>MKHHHHHHMHAGAQMDAESIEWKLTANLRNGPTFFQPLADSIEPLQFKLIGSDTVATAFPVFDTKYIPDSLINYLFKLFNLEIESGKTYPQLHSLTKQGFLNYWFHSFAVVVLQTDEKFIQDNQDWNSVLLGTFYIKPNYAPRCSHNCNAGFLVNGAHRGQKVGYRLAQVYLNWAPLLGYKYSIFNLVFVTNQASWKIWDKLNFQRIGLVPHAGILNG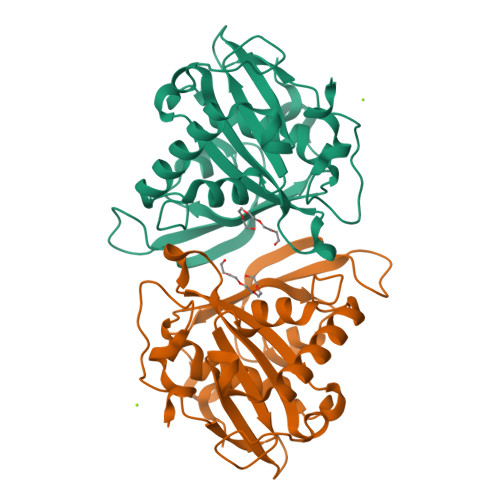FSEPVDAIIYGKDLTKIEPEFLSME[3x]>MKMEARQKQNSFTSKMQKIVNHRAFTFTVIALILFNALIV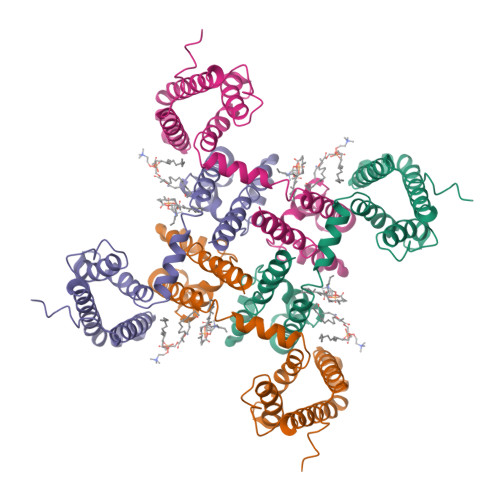GIETYPRIYADHKWLFYRIDLVLLWIFTIEIAMRFLASNPKSAFFRSSWNWFDFLIVAAGHIFAGAQFVTVLRILRVLRVLRAISVVPSLRRLVDALVMTIPALGNILILMSIFFYIFAVIGTMLFQHVSPEYFGNLQLSLLTLFQVVTLESWASGVMRPIFAEVPWSWLYFVSFVLIGTFIIFNLFIGVIVNNVEKAELTDNEEDGEADGLKQEISALRKDVAELKSLLKQSK[4x]> MTGMTNVTKLAS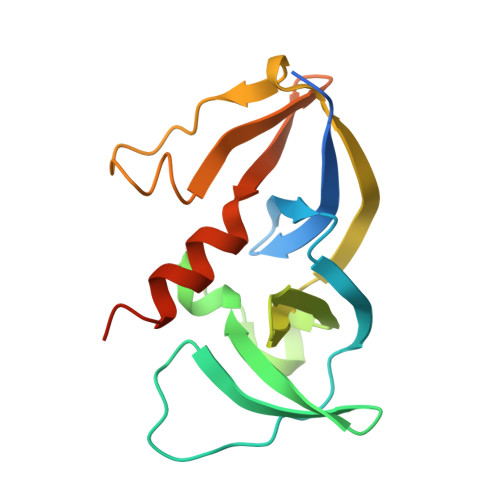EPSGQEFLVFTLGDEEYGIDILKVQEIRGYDQVTRIANTPAFIKGVTNLRGVIVPIVDLRIKFSQVDVDYNDNTVVIVLNLGQRVVGIVVDGVSDVLSLTAEQIRPAPEFAVTLSTEYLTGLGALGDRMLILVNIEKLLNSEEMALLDSAASEVA>[3x]MVVGWHRPTRLHIDTQA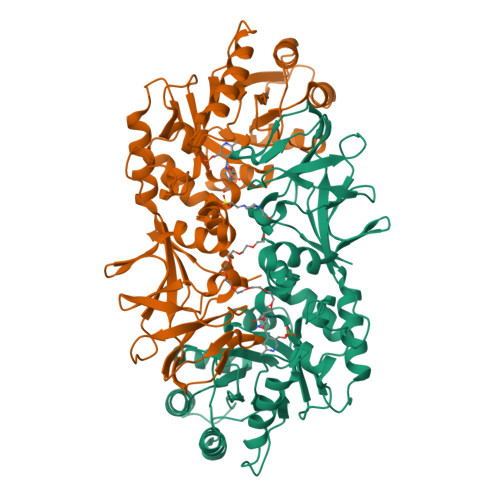ITENVQKECQRLPEGTALFAVVKANGYGHGAVESAKAAKKGGATGFCVALLDEAIELREAGVQDPILILSVVDLAYVPLLIQYDLSVTVATQEWLEAALQQLTPESNTPLRVHLKVDTGMGRIGFLTPEETKQAVRFVQSHKEFLWEGIFTHFSTADEIDTSYFEKQAGRFKAVLAVLEELPRYVHVSNSATALWHPDVPGNMIRYGVAMYGLNPSGNKLAPSYALKPALRLTSELIHVKRLAAGEGIGYGETYVTEAEEWIGTVPIGYADGWLRHLQGFTVLVNGKRCEIVGRVCMDQCMIRLAEEVPVGPVVTLVGKDGNEENTLQMVAEKLETIHYEVACTFSQRIPREYN2,8-dithioxo-1,2,3,7,8,9-hexahydro-6H-purin-6-one 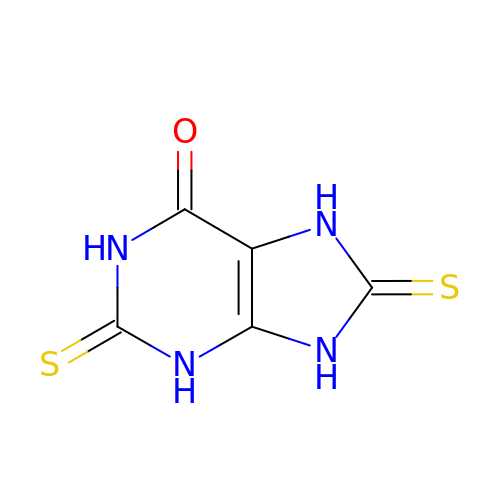| C5 H4 N4 O S2 | NDSUZZIWNBVBKW-UHFFFAOYSA-N> QGFSLAQYLQEQKTIVETALDQSLVITEPVTIYEAMRYSLLAGGKRLRPILCLAACEMLGGTAAMAMNTACALEMIHTMSLIHDDLPAMDNDDLRRGKPTNHKVYGEDIAILAGDALLSYAFEYVARTPDVPAERLLQVIVRLGQAVGAEGLVGGQVVDLESEGKTDVAVETLNFIHTHKTGALLEVCVTAGAILAGAKPEEVQLLSRYAQNIGLAFQIVDDILTYPSLWGIEKSQAEAQKLVAEAIASLEPYGEKANPLKALA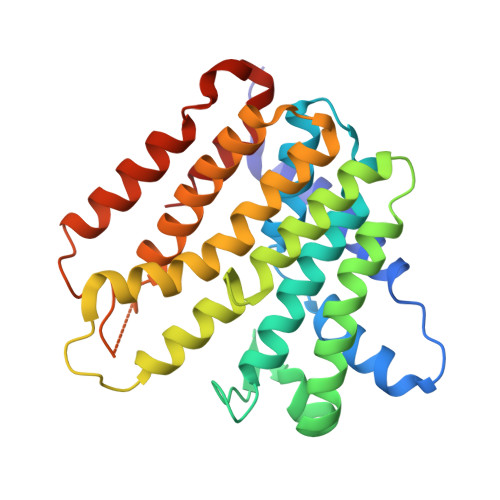EYI P1-(5'-ADENOSINE)P4-(5'-URIDINE)-BETA,GAMMA-METHYLENE TETRAPHOSPHATE | C20 H29 N7 O20 P4 | 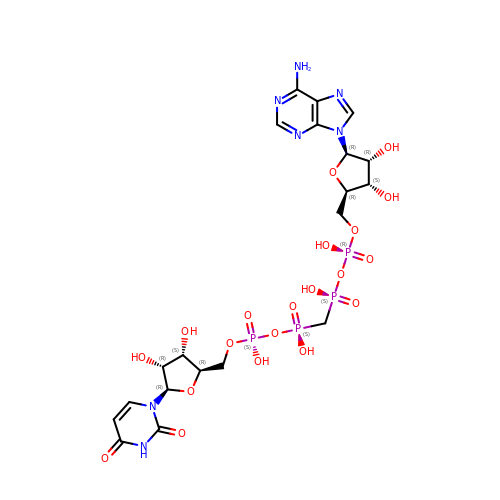CDWUJMZPKJSQNK-LKAJGUBRSA-N>MEFNNTIPELVCRDIDSSLSFYTQKLGFKVLFEREEQGFFFLYKNDIQLMLQQLGETAWMSHSNDTPFGNGMNIAFKVESLDDLDCS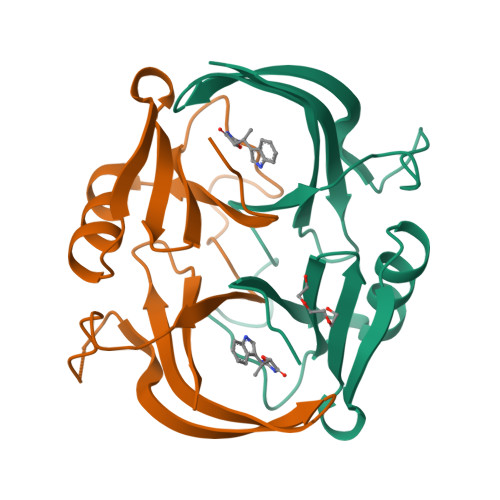TPSEDIFLETETIEYRVLDGVASVNQVIFRDPDGYLIRFVEQVNQLEHHHHHH[2x]>[2x]MHISDEQLKRPLRDYGEALEMWSTFQTKTQALSQSLSSQLRLILTGSGIPSKRAYQILLCVDDSSSMSDDNRSTAGNLALESLVMVARALTVLEAGQIGVMGFGTDVFVAHALTDPPFTSQDAGARVLQQFTFRQDSTDMVLLLRRTIDHFREARLIQASSSRGGEDLWQLALILSDGLVQSRDHARLRPLLREAMEQRVMVVFIVMDDARSRKGHSVLELKEARFGPDGVPVIHRYLDSFPFPYYLIVHHLEDLPGALAALLRTWFAEVNSGSHHHHHH;>[2x]MKHHHHHHPMAPAPVAQVKVIFTTTEPDLELPESKRQLLVPADIRRYGLSRILNSESMLDTGSIPFDFLINGSFLRSSLEDYLTSNGLSLETTLTLQYVRS

One of these energy-consuming enzymes is the conserved huge AAA+-type ATPase Rea1 (also known as Mdn1), which is composed of a hexameric AAA+-ATPase domain, followed by a long tail consisting of an α-helical linker region, a flexible aspartate/glutamate (D/E)-rich domain and a C-terminal metal-ion-dependent adhesion site (MIDAS) homologous to the inserted (I) domain within the α-subunits (αI) of integrins that mediate ligand recognition. The conserved interaction between the C-terminal Rea1-MIDAS and the Rsa4-UBL (ubiquitin-like domain) or Ytm1-UBL is essential for assembly of the 60S pre-ribosome in a reaction mediated by the Rea1 ATPase upon ATP hydrolysis that leads to the removal of Ytm1 and Rsa4 from distinct pre-60S intermediates. In this study, we report crystal structures of the Chaetomium thermophilum (Ct) Rea1-MIDAS, both alone and in complex with its pre-ribosomal substrates, the CtYtm1- or CtRsa4-UBL domains. Besides displaying the typical MIDAS fold known for integrins, the CtRea1-MIDAS crystal structures reveal evolutionary conserved Rea1 specific structural elements.

Next, we aimed to structurally investigate the complex between CtRea1-MIDAS and its two ligands, the ubiquitin-like domains (UBL) of CtRsa4 and CtYtm1. However, purification and crystallization proved to be challenging and might have been impeded by the conserved but flexible MIDAS loop (element II). Since this loop (deletion of amino acids 4734–4773 in CtRea1, or 4657–4696 in ScRea1) is dispensable for MIDAS–Rsa4 interaction, we replaced it with a short Gly-Ser-Gly linker. Using these trimmed constructs, we were able to reconstitute the complexes CtRea1-MIDAS∆loop–CtRsa4-UBL and CtRea1-MIDAS∆loop–CtYtm1-UBL, which readily crystallized, allowing us to solve their crystal structures at 1.89 and 1.84 Å, respectively. Although the overall structures of the Rea1-MIDAS ∆loop domain in complex with either Rsa4-UBL or Ytm1-UBL are highly similar to the MIDAS apo structure, the terminal helices α1 and α9 were slightly tilted (as observed upon binding of integrins to its ligands for the C-terminal helix). The Mg2+-binding site in this case is fully ordered and the metal ion is coordinated cooperatively by the MIDAS and UBL domains. However, one unforeseen major structural re-arrangement concerns the Rea1-specific element III, which in the apo structure forms a loop that crawls along helices α1 and α9 and was not fully resolved, but in the ligand-bound form becomes re-arranged, the short helix α8 partially unfolds and forms a β-hairpin that provides an additional binding site for the UBL domains of Rsa4 and Ytm1. To assess the functional relevance of the Rea1-MIDAS β-hairpin–UBL interactions, we performed genetic interaction studies with Rsa4 and Ytm1. The combination of the rea1 Y4859 > A/R I4871 > A/R constructs with mutant alleles of either Rsa4 (rsa4-1) or Ytm1 (ytm1 S78L)25,38 yielded cells, which were no longer viable.>EKQLMNVEPIHADILLETYKRKIADEGRPFLAEFQSIPRVFSKFPIKEARKPFNQNKNRYVDILPYDYNRVELSEINGDAGSNYINASYIDGFKEPRKYIAAQGPRDETVDDFWRMIWEQKATVIVMVTRCEEGNRNKCAEYWPSMEEGTRAFGDVVVKINQHKRCPDYIIQKLNIVNKKEKATGREVTHIQFTSWPDHGVPEDPHLLLKLRRRVNAFSNFFSGPIVVHSSAGVGRTGTYIGIDAMLEGLEAENKVDVYGYVVKLRRQRCLMVQVEAQYILIHQALVEYNQFGETEVNLSELHPYLHNMKKRDPPSEPSPLEAEFQRLPSYRSWRTQHIGNQEENKSKNRNSNVIPYDYNRVPLKHELEMSKESEHDSDESSDDDSDSEEPSKYINASFIMSYWKPEVMIAAQGPLKETIGDFWQMIFQRKVKVIVMLTELKHGDQEICAQYWGEGKQTYGDI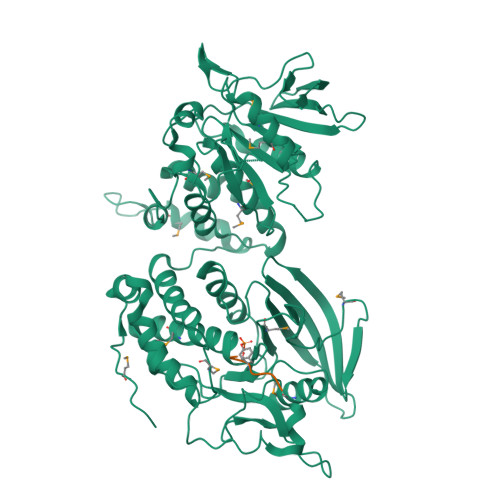EVDLKDTDKSSTYTLRVFELRHSKRKDSRTVYQYQYTNWSVEQLPAEPKELISMIQVVKQKLPQKNSSEGNKHHKSTPLLIHCRDGSQQTGIFCALLNLLESAETEEVVDIFQVVKALRKARLGMVSTFEQYQFLYDVIASTYPAQN[2x];>[2x]REEYDV> MKRILLVLLTLVFLGAIACQRKEENKTEMVKLKRMIAQFAPTEIKYDHSLLDERKQKVVENLYRAAKIMDEIFLDQVYSKNFEIREQLRASSDPLDQLRLEYFTIMFGPFDRLNHDKPFIGNTPKPKGANFYPPDMTREEFENWLKAHPEDEAAFTSEFTVIRRQDGKLVAIPYSEYYKEYLTRAADYLKKAAEFADNPSLKKYLQLRAEAFLNNDYYESDLAWMDLNDHTIEVVIGPYEVYEDKLFNYKAAFEAFITLRDPVESAKLKKFVGYLDEMEKNLPIPDAYKNFNRGSESPMVVVQEVFSAGDTKAGVQTLAFNLPNDERVREAKGSKKVMLKNIHEAKFDKLLKPIAEKVLFAEQLPLVTFEGFFNHTLMHEISHGLGPGKIVLNGRQTEVKKELKETYSSIEECKADVLGMYNNLFMIEKGVYPPEFEKQIYVTFLAGIFRTIRFGINEAHGAGNAVIFNYLLEKGAYQFDPAAHRVKVNFEKIKDGVRDLANKVLTIQAQGDYMAAKNLLETYAVESEPIMIMRARLQELPVDIKPIFQIEKELGNSNLEHHHHHH

DPP III (EC 3.4.14.4) is a cytosolic zinc-metallopeptidase which cleaves dipeptides from the N-termini of its substrates, consisting of three to ten amino acids. However, they enabled the recognition of five evolutionary conserved amino acid sequence regions in the M49 family, including the unique hexapeptide zinc-binding motif HEXXGH. Furthermore, this is the first functionally and structurally characterized member of this family with hexapeptide M49 signature motif reduced to the pentapeptide HEISH.

CaDPP III is much shorter (558 amino acids) than the already reported human (737 amino acids), yeast (711 amino acids) and B. thetaiotaomicron DPP III (675 amino acids). Similarly to the other available crystal structures of M49 family enzymes, the structure of CaDPP III consists of two structural domains, called upper (containing zinc ion) and lower domain, which are separated by the inter-domain cleft. The zinc ion, essential for the enzyme activity, is positioned in the lower part of the upper domain where it is pentacoordinated by two histidines from the first conserved, zinc binding, motif H379EISH, one glutamic acid (E442—bidentately) from the second motif E441ECKAD and a water molecule. Although CaDPP III has shorter first conserved motif, pentapeptide vs hexapeptide, there is no significant difference in the zinc binding site in these two orthologs. Although smaller than the other DPPs III, the CaDPP III lower structural domain core is also comprised of five-stranded β-barrel surrounded by α-helixes. The crystal structure of CaDPP III is very compact and more similar to the closed B. thetaiotaomicron and human DPP III forms than to the open ones. The conformation of CaDPP III is partially closed, probably due to the Ala-Lys dipeptide bound into the protein active site. Since Ala-Lys was never added to the crystallization solution, we assume that it was bound into the inter-domain cleft during protein expression. However, the lower CaDPP III domain is 85 amino acid residues shorter and lacks the α-helix-loop-α-helix motif, two β-strands, and α-helix at C-terminus. The finding that the relative number of non-covalent interactions within CaDPP III is larger, while the share of loops (unstructured regions) is lower than in its mesophilic counterparts suggests higher rigidity and compactness of this enzyme, and gives possible explanation for its thermal stability.>[2x]GEIRPTIGQQMETGDQRFGDLVFRQLAPNVWQHTSYLDMPGFGAVASNGLIVRDGGRVLVVDTAWTDDQTAQILNWIKQEINLPVALAVVTHAHQDKMGGMDALHAAGIATYANALSNQLAPQEGMVAAQHSLTFAANGWVEPATAPNFGPLKVFYPGPGHTSDNITVGIDGTDIAFGGCLIKDSKAKSLGNLGDADTEHYAASARAFGAAFPKASMIVMSHSAPDSRAAITHTARMADKLR

NDM-1, as a typical member of B1 class of MBLs, possesses two Zn(II) ions intercalated by a nucleophile hydroxide in its active site, which is delimited by flexible loop 3 and 1023. The two Zn(II) ions have been validated to be crucial for its hydrolytic activity to launch a nucleophilic attack on β-lactam rings in β-lactam antibiotics. The Zn(II) ion in the active site of MCR-1 has been validated to be vital for the PEA transfer process; notwithstanding its biological roles in MCR proteins are still controversial. Our results showed that AUR irreversibly inhibit NDM-1 activity and disrupted the function of MCR-1 via displacing Zn(II) ions in the active sites and thus forming Au-NDM-1 or Au-MCR-1.

Au-bound NDM-1 was first obtained by incubating apo-NDM-1 with 10 molar equivalents of AUR overnight at 25 °C and then co-crystallized using a typical sitting-drop vapor diffusion method. Two Au ions, viz, Au282 and Au283 were clearly observed in the active site, tetrahedrally coordinated to Cys208, His250, Asp124, a water molecule (w291), and His122, His120, His189, and a water molecule (w410), respectively. The distance between two Au ions (~3.8 Å) is much shorter than that between two Zn ions (~4.6 Å) in the intact NDM-1 crystal. An additional Au ion (Au281) resided in the interface of two protein monomers coordinating to Asp223, Glu152, a water molecule, and a Glu227 from an adjacent NDM-1 molecule in a distorted tetrahedral geometry. The bond lengths of Au(I) with the side-chains of those amino acid residues were overall in the range of 1.9–2.5 Å and generally comparable to those for Zn(II). The occupancies of the three Au ions were ca. 0.5 with the Au283 in the Zn1 site showing slightly lower occupancy (0.45). The active-site pocket of NDM-1 in the crystal structure was widely open and two Au ions resided in the bottom of the cavity, apparently being assessable to AUR. Overall, the data agreed well with our biophysical characterization that the Zn-dependent hydrolysis function of NDM-1 was inhibited by AUR through displacement of the Zn(II) in the active. Our crystallographic analysis confirmed the binding of Au(I) species to the cysteine residue at the active site of NDM-1. Unlike bismuth, each AUR displaces one Zn(II) and tetrahedrally coordinated to respective three residues in either Zn1 or Zn2 site of NDM-1.> GPLMSGLNDIFEAQKIEWHEGSAGGSGHMTDLRKLEALQALHAELVAVRQHRFEGLQVLETLLEEQTDAFKALIAKPARDTKDREALGKEPKKLKIGEEEYSLNEDFVNDCLKLADELDLNEKESARILIDCDAEGDVETQSRPLWECGVIRFHQERKYLLDCMRLILEIAADEDIDAGLQESFGVAAEDKIFGIPPPWERNKENQPTQVKKFIPRCMEAMKGVRSMLQCMADKANARNMLQQASLVRPLDNQETLDFSRLSLVEQHECLASILHAAVQRHHATIADFQDFIKILRKWDKYDHFLIHLIPVLAAYITEFGSPEGMGDLQQARRLNDFICKGGDEDSWALPVLGAAVRAWWIAEHNGFYLDDTVQDLRGINLDEEDEQRTKQFLDALKEGAFDFILSVAADCKAQEWQDPSQLGARQWLQRKIPSLPSEPFPFSHFLQHSLMVHLEGFVDATISNLPDVLRKLRTEEDEQRQLRPNHEQDMDLERFLIIISYAYEGRPDAAMSFWEDPDSNLAGFLQWASRRASTPLVSAFCEMLRCLADNEECATAAHNFLLDEGHQASGKMKRSQSLTWSQIFKELEYFTTKVCSERPNPPQASMHRPGRPGADPAEIEPESALMLECYLRLIAKLATESEIARKRLIMDEDFNLVDTILKLSVGVIPHRLRACIFYVLKALMIRKTHEELDAMWRWVEAWMTNPFSSLPGSQGAPQRISFLGQTPGPQECMEMMFREFGTGFEQSNAFIQLLTTLLVPPEGLNSLNDSVPFPEWLGSSIRTLGIEPYVDFVFDVFANRTKDISDPSQLRILRLSCLDFVMVCLVTFNEDLIVLGHESNISIDDAMAATNLATYVRLHPFSRVMEWLFNEKVITSLINTIHQDPISLGSASPDSPLVVSILRAIQVMIKALELQETYLHLVRPEVLRYQGEAGVRRKPVANAAYSAFEDGILSHLSLVVDLGKYCNLGHAELTLACLKLLEKISTSSRILSAWSPDSGRLGHRNKAIVQLERNGEGETISASLSASIMATLDPALAASGENYRVKLAILDFLYACLRATPDQPTIAHQLLGFH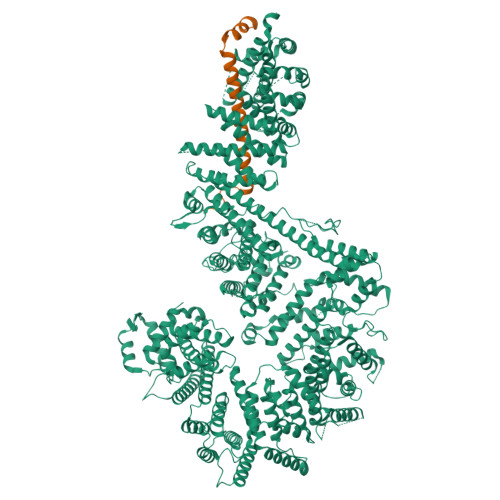CELSKLGIEPKGPFDMQKSLFHSLLNVLITLTVSEEEQGMRGYLVTLKYRVLRILQLLWKSPLSASLVMDELRATNFLFHMLLREVQIQPQLPWDGQLVTGCEFLLSDASLAYIDYLASRAAIFEYIGKELCSVSQNRIPSIKRQIFDALNGQIFVDEEAPLTIPSIFDFFDFINTDYKWEEIPSPHFTYLKDLDLGPCILEHKYAGVHYDIRKAQEILALKRKEYEHSQLATPEFLETVELEEKVLIEWLTVRNRANLLLTARLNLLQAWANLLLVMIESNDFKSTPKMAFLLQALQAILPTLEAFSSLKSDEAFELARVAKVLLWKLDFSQDSDAGLDREQFTVGNLIGDKLFQLFQLCLSAISQCSGTPELRSLYYSICYRYLTAVVDNDATVAATPASSTIGPTRSVTNARARTLKAITLYGDRLLNVICDDAYGSDTTCQTAAMILLNALVHTSRASSAAGVSPADVDCPIIDALNRLNFIGVLVDSLKEILNEWLAPSSTFDPSLSTNASPSLPIPASPSQQYTSAKLALLLQLCQTRQGAKYVLQANLFRALEQSGVFAADPELVEVDSESGVPRVVALERHYALLVALARVVGAAVTARGAHNIVQGRKFLTQHRGLVVHVLKKNAGIGGGVVGNSLASSINGGSTATMTRRDEILAQQALEERIEELAEAFMLLITATGFLEYESEQVPSEQPRAHTTFFH;> SGTGLGEVDVDTYLSNLQTKTTLSMIADGLERSARDFDAFLEENVTLEWEAQRKRIYQHFGIK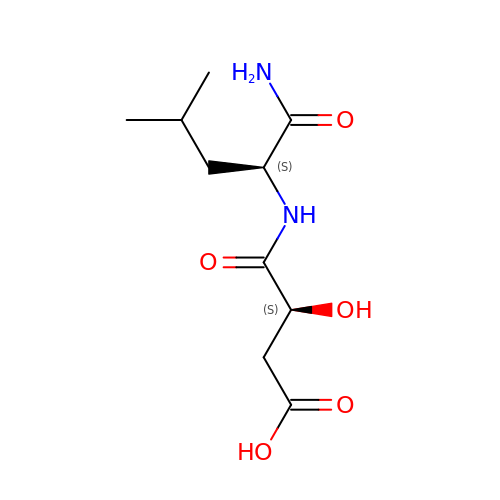(3S)-4-{[(2S)-1-amino-4-methyl-1-oxopentan-2-yl]amino}-3-hydroxy-4-oxobutanoic acid | C10 H18 N2 O5 | LHEOILLGVMWLIK-BQBZGAKWSA-N>MGHHHHHHAENLYFQGHMHKVKLAAITCELPARSYENDDPVFAAVPDLSESWWQFWGVNRRGYFDPRNGENEFSLVVRAAERLLRSSDTAPDSVDMLICSASSPIMTDAGDVLPDLRGRLYPRMANVLSKQLGLSRALPLDSQMEAASFLLNLRLAASMIRQGKAEKVLVVCSEYISNLLDFTSRTSTLFADGCAVALLTRGDDDSCDLLASAEHSDATFYEVATGRWRLPENPTGEAKPRLYFSLFSDGQNKMASFVPTNVPIAMRRALEKAGLGSDDIDYFVFHQPAPFLVKAWAEGIGARPEQYQLTMGDTGVMISVSIPYTLMTGLREGKIRPGDRIVMAGAATGWGFAAQVWQLGEVLVC[8x];>MLIQAVGVNLPPSYVCLEGPLGGERPRAQGDEMLMQRLLPAVREALDEAAVKPEEIDLIVGLALSPDHLIENRDIMAPKIGHPLQKVLGANRAHVFDLTDSSLARALYVVDTLASDQGYRNVLVVRGESSQGLEVDSESGFALADGALALLCR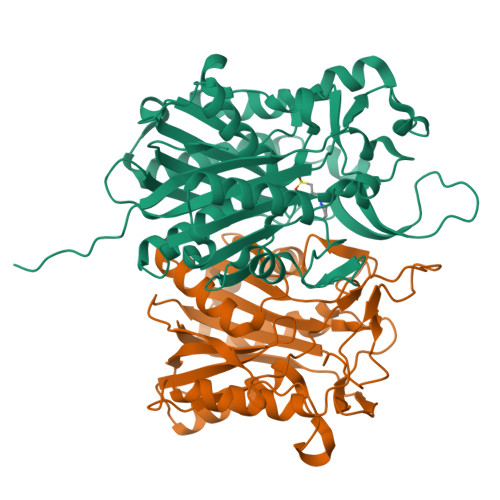PTGKAAFRRGALGGDPAQEWLPLSIPLNTDIRQVGDVKGHLNLPAQPGLPEAVRAGFTRLAGDFPQLNWVREEWFGQGRPDGRCLGPFELASQLRAAQRDRLDELLLISFDPFGMVVEGVTLELAGEAHA[8x]2'-deoxy-5'-uridylic acid | C9 H15 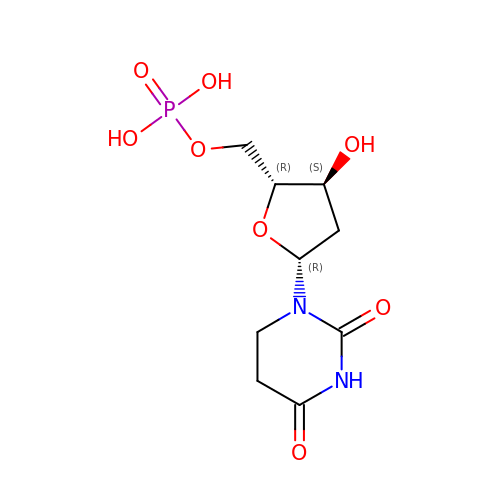N2 O8 P | WQQZADPPRABIFU-SHYZEUOFSA-N> GLPTMNTPGSCQFLTSDD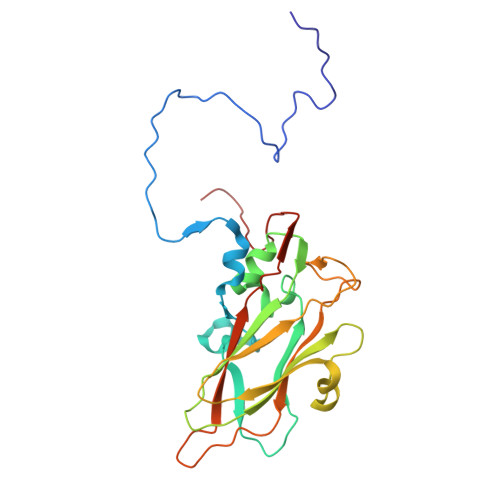FQSPSAMPQYDVTPEMRIPGEVKNLMEIAEVDSVVPVQNVGEKVNSMEAYQIPVRSNEGSGTQVFGFPLQPGYSSVFSRTLLGEILNYYTHWSGSIKLTFMFCGSAMATGKFLLAYSPLGAGAPTKRVDAMLGTHVVWDVGLQSSCVLCIPWISQTHYRYVASDECTAGGFITCWYQTNIVVPADAQSSCYIMCFVSACNDFSVRLLKDTPFISQENFFQ>MAAFSAINVEPEDNVDEEYDTTKEVQVEEALKLFQTALKLHAQGPQFFDQASRAYAALFQSEIFKYPESKTDYERAEAGQDVAAAAFIPGVEILGADIDGASTLPQTFYLSYKNHGQFILDRIKHRTRTENIGKEELLNDADVRKDAYQALYNFCVALDRDPSDADLWRKAARLAAFLRSPRITRYSLEAAIEMDDDPAVDEVNPPSLAEGFAGEQLKQQLQVLDDKIALTHPIMKPFLEKDIPPYLAEYLDPMPFLPDPSKQLAVPGQQSPSVENARLTIGLSNISWTELGTALVNLAKEEGLSSKGISIQLPATSSDEDVQMEVDAQLQLPKSQPPPAQLDVGQVDGDNTEHPAEVGVKVEEPEPAELEPASANDESSKDQGSSRKRSQSAAGIPDTQEDEAADLKRSKRTRRRDTTADEAMDSATFFATQLQPLQAADQNLFQATKNLLENLGVTDRVTLDRIAEVLDSCASDDRTSKFQNPATVDLRNALMNFDEDVAAILLNQRELPQLNLSTFLEHAKSGSQRALEAPAFDDARGLRGFVERLGDAWNTIHDVAYGYVKALADFYTDFKWSEPLRATVIQLINSLDSSIYDGIVHDLEACQSITKDSSFSKLASLAQMLLELHLDVLDRVNESNGSAEEITKVEAKGRLRRWMELVTKVLRMRDLEQAGTLPLRYLWAAVTSTTLAKEAPREHILNCWYSLRDYLTGSVSAEISLPNNSVMPEISLSAADREISKLTTMDFFLGIFQEEMSDPVSVIENLEPVLSPESVQICVPVSETDSLENSNDTSKSKVKKLPITECASQELLDLWKFLNSSSTELRLLLWSRLAEAYGRIKYTTKQFSCFLRSIEVIVADFEGEEYASTPPEARKTLFMGMLKALDDLIIQSLHLALNDNSSFDIIDEDHLRSSMSAIAKVSCMLHVAAMYEDEGRIGILPSPANGSPQKSFLNKLQEMQVRTWSLQYTMLKVGINQHPDIFPKPENDLAEFLAAVHQVLGLRKCCKSSNRIFLKMMRVELLKQKNIENWEDYLGQVLYDLHGLKLGVGVWDVQDHGCEPENLEKRQALQLVEKVAMLANRMSMKDLLKSDLKTTIERMQQAIGSAKSSPQMSHNLRNYTEYLKSPIHPLHMYQALTGGVHLDAVSINTPESAPAKQGWFFLLGMIALTKFKGVDLNRRQTPGATDDLRIAATFLRLQLQYTPDRWDAWFRLAECFDYELEEAVLWTADKMNKERAELVKFQRHAIHSYIMALSHSYAWASNPAALTSLEDDEEALYDMYHEFGMRLYSSSREPFAMEPFEHGDHKRFFIEPEGAGTYKKIVHNQMTDYQVWKFAAHLFRKAMVGKPKDWKNPYMVAKCLWKMYQKPTEELDEKNRRHRPTVQMVLDALEKTIEVVSALPKPRHGQEPILEPHYKIVSVIWKLVKRGDLSPQEATKVLQRQPYSPDHGKEVSVETAEDFKAYIIRCLRYLRDKDKSNWQHRLIIRHARVLFDENTDMNRPDAVEAAKAAFGVLRENMFTKTMVMNVWKCDAERPGRHHVYTERYIRYVVKLLDVMNDRTNMGALLRRIRKKGADFYHFNELWQYCVHTYVKLLRDTFNIPVSEEDVFKTLTPEEFDVVGEKIADWAATPDAENHDALGAMKEAVELKKLNANLMKAGLIDDLIADCYTAVYSYVRPELPRPERTPLPDTTPSSPKSENVPPPPADAVDLKSRLLHTLVTRDKEPSTSSILGSLRAGSSELQDRSEKHSVAGDVPQRAHRVGVGIRRPNIIRKAEQAVQAALRAAEGAAARAGTNGSSTGPSGTKSRVGSISSLRAGRTATRGEDEEDSEGDEDGDVEMKEAEGEGPIAGRRSRRQSNATNKSTGAVADEDEASDVSSPPGSLHDSADDESELSDVPADYEDDAPPALLFPNLRRSVDAGTPGSGEEDETETEHDTGNRSGEEEEQEEEAEDGSEEGDEDAAVEDHEENEETDKGVDVEEHADDEEGEEDIEETEEQGNDGDSKVQDDAMEVEGEEAEDSEATEEGD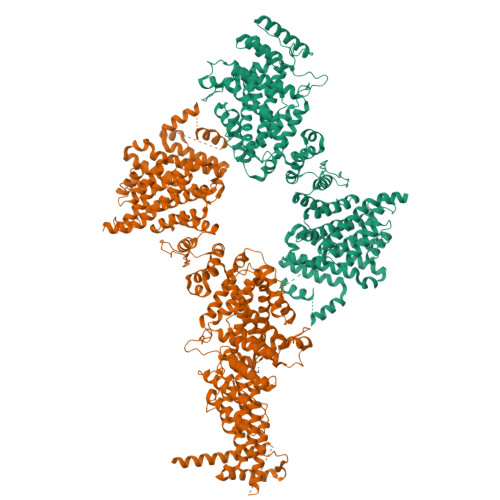DSIIFTQQNHIVTSQSEQNGVPQAHRKSPYIPMLSPAPQPILTFSQELSECTTNPPTGMTIELPNEADLHRWHVTLEGPENTVYAGGKFGIVVTLPPEYPFKAPNITFATRIYHPNVTNDSLGHICLGLLKSENWKPSTRLASVLEAVRGLLVEPQPEDPLEARIADEYRRDRKEFEKNARTYVQRYAKGPVKWEDSVTSTTTASSGSS[2x]> MAASRRLMKELEEIRKCGMKNFRNIQVDEANLLTWQG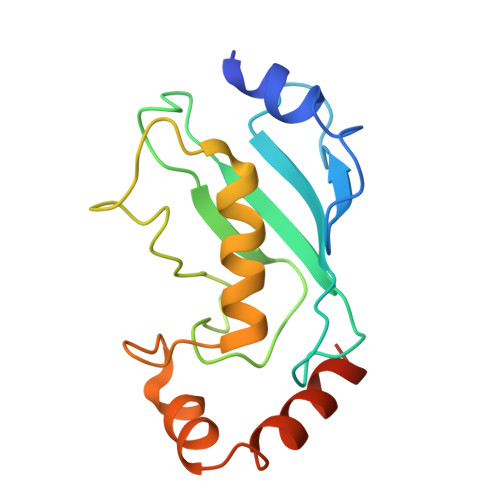LIVPDNPPYDKGAFRIEINFPAEYPFKPPKITFKTKIYHPNIDEKGQVCLPVISAENWKPATKTDQVIQSLIALVNDPQPEHPLRADLAEEYSKDRKKFCKNAEEFTKKYGEKRPVD>CGTTAATTA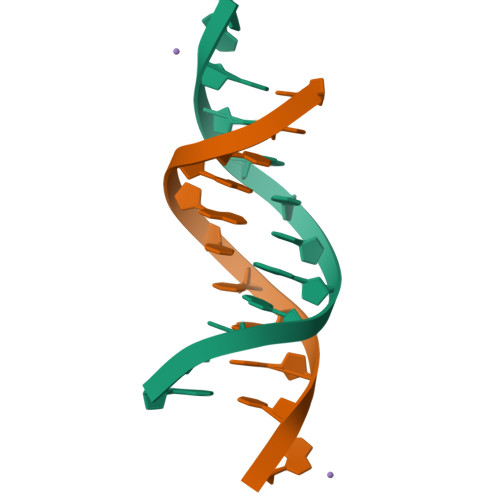ACG[6x]(4~{S})-4-azanyl-5-oxidanyl-pent-1-en-3-one 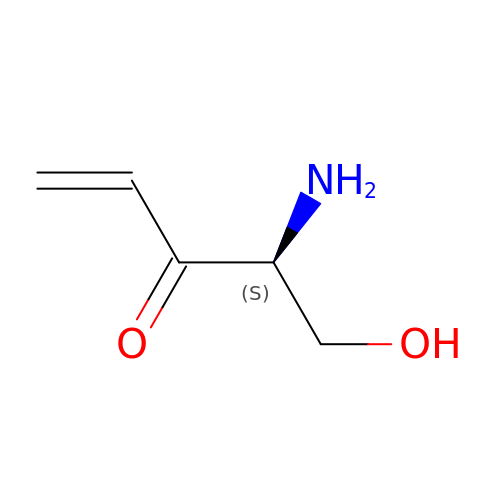| C5 H9 N O2 | UCJPATVGPSMUQX-BYPYZUCNSA-N1-{(1S,2S)-1-(2,4-difluorophenyl)-2-[2-(3-methyl-1H-pyrazol-5-yl)-4-(trifluoromethyl)phenoxy]cyclopropyl}methanamine | C21 H18 F5 N3 O | 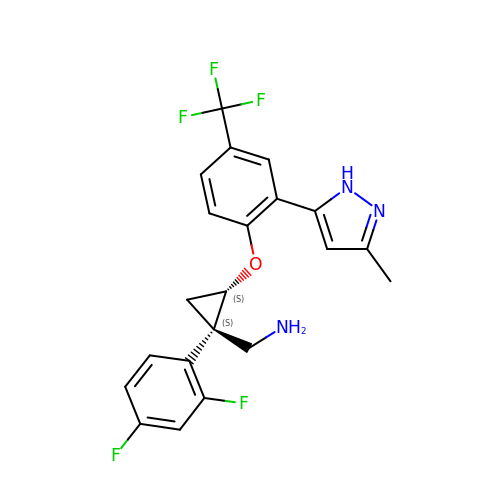GGPJTWFNIVZVBE-VQTJNVASSA-N>[2x]MAGTGHTPEEALALLKRGAEEIVPEEELLAKLKEGRPLTVKLGADPTRPDLHLGHAVVLRKMRQFQELGHKVVLIIGDFTGMIGDPSGRSKTRPPLTLEETRENAKTYVAQAGKILRQEPHLFELRYNSEWLEGLTFKEVVRLTSLMTVAQMLEREDFKKRYEAGIPISLHELLYPFAQAYDSVAIRADVEMGGTDQRFNLLVGREVQRAYGQSPQVCFLMPLLVGLDGREKMSKSLDN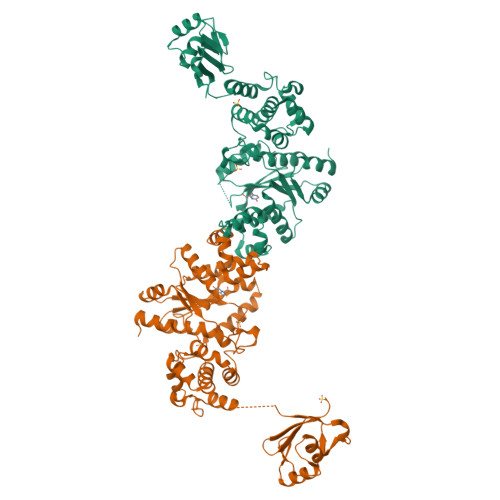YIGLTEPPEAMFKKLMRVPDPLLPSYFRLLTDLEEEEIEALLKAGPVPAHRVLARLLTAAYALPQIPPRIDRAFYESLGYAWEAFGRDKEAGPEEVRRAEARYDEVAKGGIPEEIPEVTIPASELKEGRIWVARLFTLAGLTPSNAEARRLIQNRGLRLDGEVLTDPMLQVDLSRPRILQRGKDRFVRVRLSD>[2x]HGHHSHGKPLTEVEQKAANGVFDDANVQNRTLSDWDGVWQSVYPLLQSGKLDPVFQKKADADKTKTFAEIKDYYHKGYATDIEMIGIEDGIVEFHRNNETTSCKYDYDGYKILTYKSGKKGV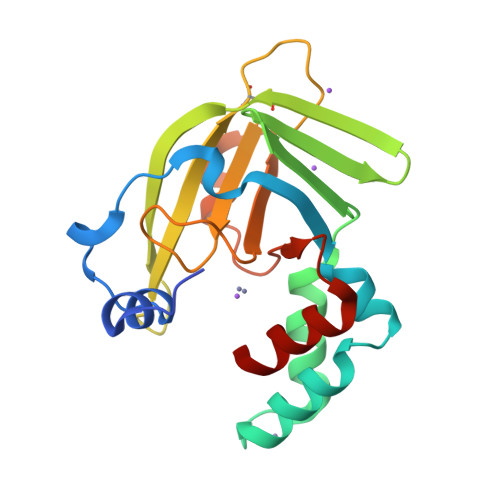RYLFECKDPESKAPKYIQFSDHIIAPRKSSHFHIFMGNDSQQSLLNEMENWPTYYPYQLSSEEVVEEMMSH1-MYRISTOYL-2-MYRISTOLEOYL-SN-GLYCERO-3-PHOSPHATE 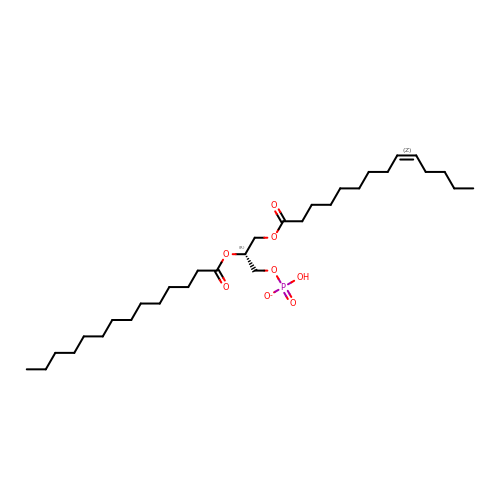| C31 H58 O8 P | GVANAVLIALOKCA-HQGHLRICSA-M> EFALLTCRLDPPSQDLKDGTQEEATKRQEAPVDPRPEGDPQRTVISWRGAVIEPEQGTELPSRRAEVPTKPPLPPARTQGTPVHLNYRQKGVIDVFLHAWKGYRKFAWGHDELKPVSRSFSEWFGLGLTLIDALDTMWILGLRKEFEEARKWVSKKLHFEKDVDVNL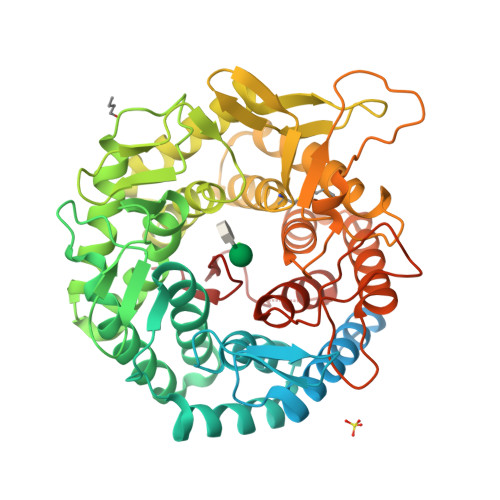FESTIRILGGLLSAYHLSGDSLFLRKAEDFGNRLMPAFRTPSKIPYSDVNIGTGVAHPPRWTSDSTVAEVTSIQLEFRELSRLTGDKKFQEAVEKVTQHIHGLSGKKDGLVPMFINTHSGLFTHLGVFTLGARADSYYEYLLKQWIQGGKQETQLLEDYVEAIEGVRTHLLRHSEPSKLTFVGELAHGRFSAKMDHLVCFLPGTLALGVYHGLPASHMELAQELMETCYQMNRQMETGLSPEIVHFNLYPQPGRRDVEVKPADRHNLLRPETVESLFYLYRVTGDRKYQDWGWEILQSFSRFTRVPSGGYSSINNVQDPQKPEPRDKMESFFLGETLKYLFLLFSDDPNLLSLDAYVFNTEAHPLPIWTPA>[4x]MADEK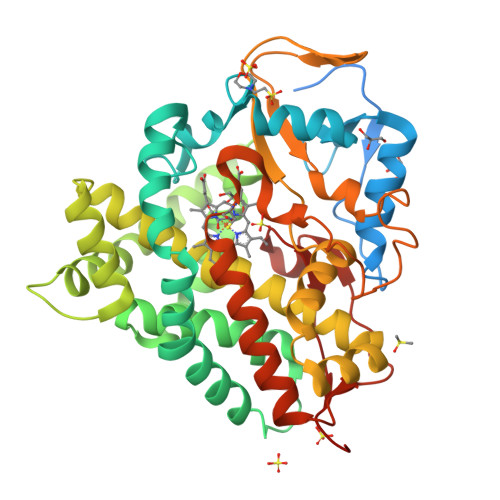APEREHNQGARADGERSSGAARRVAAFAAALPRLTLHDDLHSVSSMDFPLANLFFVPSEDATAFGRRLRAAAQQAPIVFDTAFGMPILLRKSHITTAYRDTATFSTRMFQAGILNGGLAAMQGDEHARMRRVYNMFFLPRAVSQYEERFVRPISEQVVDRLAGKPRVDLLEDFAMELPRRVIGELFGFPAEKLHETDERVRAMLRGLVRMHDPAAVAESQRAYGETLGLITEVVERESRDTSDTLLGEILRTLKAEHMDTIEASRQIVLSLILGGYETTSWLVANTIHALLAHPDTLARVRQDPSLLPAAIEEGMRWCPSSFGVLRMVERDVRLDDQALSAGTVVCLAGIAGNYDETAYPSPEVYDIDRKPLPAANVFGGGAHFCVGAPLARMEARVGLQALLARFPGLRAVPEERPSFMYGAKDSVAHGPDKLPVLLHHHHHHH>MTITANKRHYLEKVSHQGIISALAFDQRGALKQMMAAHQEGEATVTQIETLKVLVSEELTPYASSILLDPEYGLLATKVRANQTGLLLAYEKTGYDATTTSRLPDCLVEWSVKRLKAAGADAIKFLLYYDVDGDEQINLQKQAYIERIGSECTAEDIPFFLELLSYDERISDNNSAAYAKLKPHKVNGAMSVFSDKRFGVDVLKVEVPVNMAYVEGFTEGEVHYSQAEAIKAFQDQEAASHLPYIYLSAGVSAKLFQETLY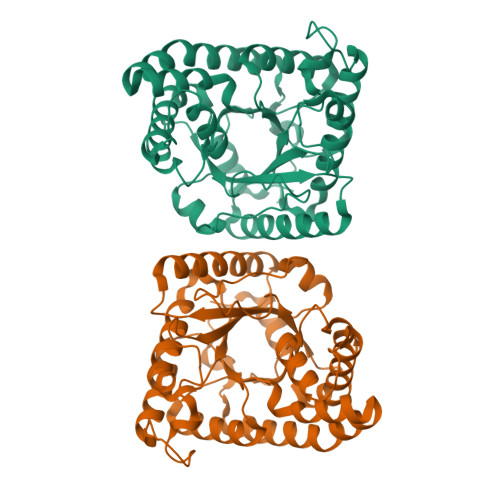FAAAAGAQFSGVLCGRATWAGSVPVYITKGEDEARKWLCTEGFQNIDELNRVLEETASPWTEKILEHHHHHH[2x]> CPERELQRREEEANVVLTGTVEEIMNVDPVHHTYSCKVRVWRYLKGKDIVTHEILLDGGNKVVIGGFGDPLICDNQVSTGDTRIFFVNPAPQYMWPAHRNELMLNSSLMRITLRNLEEVEHCVEE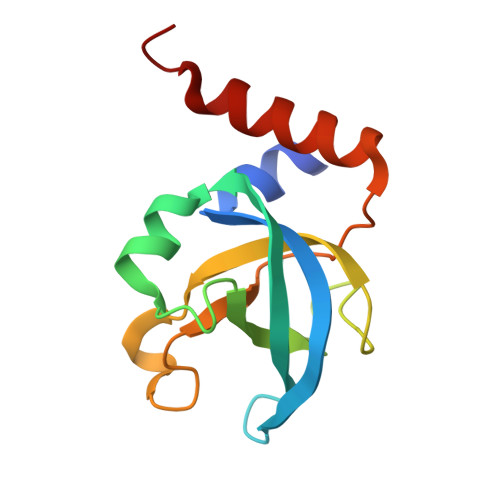HRKLLA>MSVSYETFLNKDPLDKYEDSEIYTKEWLPKVEKYRQDLKDAIPKNYTIELPKPIDDLIKDQFNAVDYLYSQKLLTPEEFAITDLSATELAKKIAAGELSSVEVFKAFAHRATLAHQFTNCAMELFIDEGLKQAEERDNYFKEHGKTVGPLHGIPISLKEQMNYKDKITHGGYVSKIVNIPNSHGVTTSILEKLGAVFYVRTSQPQTLMHLDSANNFTGLTKNPFNLLLSSGGSSSGEGAIVGYGGSAIGVGSDIGGSIRAPAAYSGCHGLRPTTKRISVKGGVSSGAGQESVPAVAGPMARSIDDLELWMKAYINEGKPWESDSTSLPMPWRDVSTPKIGDLTVAIIRDDGLVRVSPPIRRALNTVVEKLKGAGAKIIEFDPPNTKLAYETVHKMYNCDGNHMQRKLLSGSNEPLTKLTKWNLNYGEGAKHYDVASNRELNVTRDQLRDQYNDFMVQNKVDFILSPTYNNVAPHSEEVYNWSYTSLWNILDFPT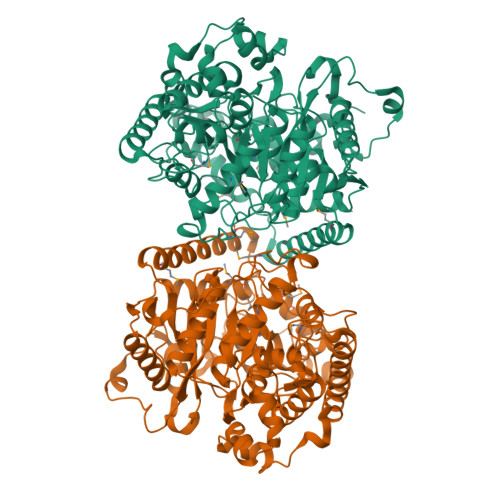LSFQTGIFQDPTKDKWTEEDTKYKYRSKLEQLENENYDPSQFVGAPVGLQLSGKRYFDEEVLAAGKAIVDLLGVDLY[2x]>SNAMSDTLYIKMDQAVEITKKQVTVGDVAKLQCKNKNITNRLKSMKLLEDTTKGK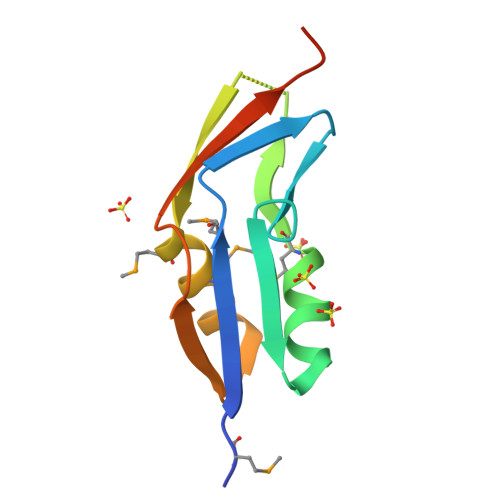KRYIVSIMKIIEMADQTFQNVDIQNIGETECVVEFKTPKKDDGPM[8x]Many folds, spanning all levels of complexity (fibrous, solenoid, toroid, and globular), clearly originated in this way. β-Propellers offer an attractive model system to study this process. They are toroids formed by sequential supersecondary structure units of typically 40–50 residues, each consisting of four anti-parallel β-strands. The units are arranged radially, with their strands perpendicular to the plane of the toroid, and have a right-handed twist, hence the name ‘propeller’ for the fold and ‘blades’ for the repetitive units. Since none of our single-bladed PkwA constructs were folded, we turned our attention to another highly symmetric β-propeller of the WD40 family, found in the C-terminal part of Npun_R6612 from the multicellular cyanobacterium Nostoc punctiforme PCC 73102 and referred to henceforth as WRAP (WD40-family Recently Amplified Propeller; ACC84870.1). WRAP, which we identified during a systematic bioinformatic survey of β-propellers, was particularly interesting in that its 14 blades are practically identical, having acquired only 10 point mutations over 563 residues (6 of these being Trp → Arg mutations at the same position of blades 1, 3, 6, 10, 12, and 13), as a result of 13 non-synonymous substitutions at the DNA level.

The 2-bladed construct behaved as a single species in solution, but size determination by SLS and analytical gel size exclusion chromatography did not allow us to unequivocally distinguish between a trimeric and tetrameric form. Instead, we used glutaraldehyde crosslinking to assay the oligomerization state of the assemblies, and confirmed tetramerization for the 2-bladed construct. As we anticipated from their oligomeric states, the 2-bladed and 4-bladed fragments formed 8-bladed propellers and the 3-bladed fragment a 9-bladed propeller. Instead, the packing of the blades within each fragment preserves the geometry of the 7-bladed parent, and the tension due to the mismatch between the number of blades in the assembly versus that in the parent accumulates at the interface between the fragments. In the two 8-bladed propellers, the one formed by four 2-bladed fragments absorbs the symmetry mismatch to different extent at the four interfaces, leading to a slightly oval shape and an approximate two-fold symmetry.

>GAMGSSSVWGVAFSPDGQTIASASDDKTVKLWNRNGQLLQTLTGHSSSVWGVAFSPDGQTIASASDDKTVKLWNRNGQLLQTLTGH[4x]> ALSARTQSSTGTHGGYYYSFWTDNPNTVTYTNQNAGQFSVSWSGNQGNFVGGKGWNPGAARTIKYSGTYNPNGNSYLAVYGWTRNPLIEYYIVENFGTYNPSSGATAAGEVTVDGSVYDIYTSTRTNAPSIEGTRTFQQYWSVRRNKRSSGSVNTGAHFNAWSNVGLALGSHDYQILAVEGYYSSGSATMTVS

Endo-β-1,4-xylanases (EC 3.2.1.8) of the GH11 family are capable of hydrolyzing β-1,4 glycosidic bonds between two D-xylopyranosyl residues linked in xylan polymers. Two highly conserved glutamates at the active site of GH11 xylanases trigger the hydrolysis of β-1,4 xylosidic linkages in xylan. In the first step of catalysis, the acid/base residue E180 (numbering to NhGH11) acts as an acid and protonates the xylan, while the other catalytic residue E89 acts as a nucleophile that provokes the departure of the leaving group to form a α-glycosyl enzyme intermediate. In the second step, the acid/base residue E180 act as a base and deprotonates the neighboring nucleophilic water, which attacks the anomeric carbon of the α-glycosyl enzyme intermediate and allows the product formation with β-configuration.

To study the structure function relationship of a new xylanase from the GH11 family the crystal structure of N. haematococca xylanase (NhGH11) was determined and refined to atomic resolution (1.0 Å). The overall 3D structure of NhGH11, consisting in total of 193 amino acids, is displayed in a single domain with β-jelly roll folding. Overall, the three-dimensional structure resembles a right hand with the fingers represented by two antiparallel β-sheets and a thumb loop located between strands β10 and β11. The inner antiparallel and highly twisted sheet creates a well-structured cylindrical cavity where xylan substrates bind and catalytic residues E89 and E180 are located. The catalytic residues E89 and E180 are located in the cleft with a side chain distance of ~ 10.5 Å. Inside the active site the carboxyl group of E89 (OE1) is hydrogen bonded to nitrogen (NE2) of Q139, hydrogen (HG3) of F137 and a water molecule (W49), while the second oxygen of the carboxyl group (OE2) is forming a hydrogen bond to Y80. The second catalytic residue E180 is forming hydrogen bonds to two water molecules via oxygen atoms OE1 and OE2 of carboxyl group, E180 strongly bends towards the main chain because the oxygen atom OE1 is forming a hydrogen bond with the main chain nitrogen of S75. The crystal structure refined with anisotropic B-factors to 1.0 Å resolution allowed to investigate hydrogen atom positions involved in main-chain interactions, side-chain interactions and even alternative conformations of amino acid side chains. A calculation of solvent accessibility shows that NhGH11 contains seven buried water molecules. NhGH11 is a mesophilic xylanase that can catalyze the efficient breakdown of xylan-based substrates at an optimum temperature of 45 °C and a pH of 6.0, and due to broad applications of its hydrolytic products NhGH11 can be considered for a wide range of corresponding industrial processes performed between 40 and 50 °C.>AQQICKAPSQTFPGLCFMDSSCRKYCIKEKFTGGHCSKLQRKCLCTKPC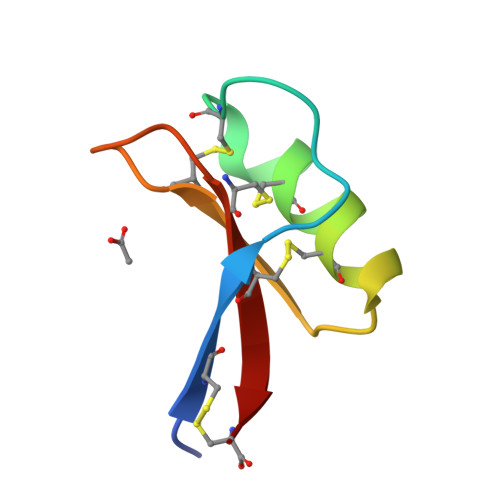[2x]> GPLGSPEFEGKITPVSVKKVDDKVTLYKTTATADSDKFKISQILTFNFIKDKSYDKDTLVLKAAGNINSGYEKPNPNDYDFSKLYWGAKYNVSISS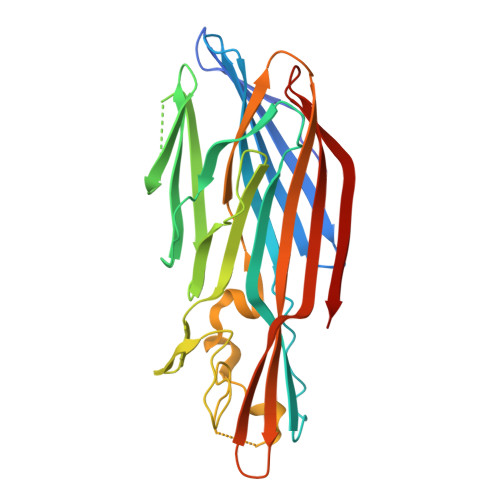QSNDSVNVVDYAPKNQNEEFQVQNTLGYTFGGDISISNGLSGGLNGNTAFSETINYKQESYRTTLSRCTNYKNVGWGVEAHKIMNNGWGPYGRDSFHPTYGNELFLAGRQSSAYAGQNFIAQHQMPLLSRSNFNPEFLSVLSHRQDGAKKSKITVTYQREMDLYQIRWNGFYWAGANYKNFKTRTFKSTYEIDWENHKVKLLDTKETENNK>MNLKV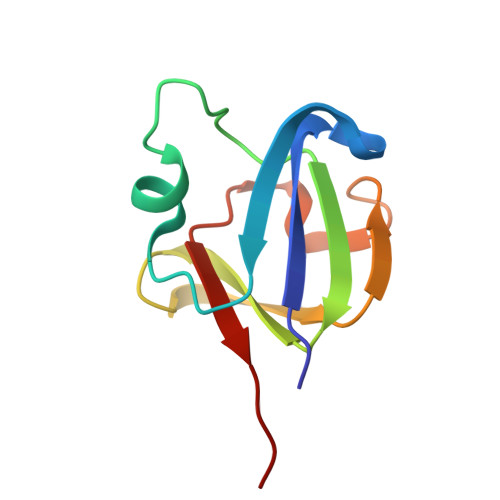ILYEKPHFLGHTKEFSEHIDSVPTFLKSDKDFHGIGSIRVIGGVWVAYEKEHFKGQQFLLEEGDFEDSSACGALSGPIMSFRYLQAN[2x]>[22x]MAALIAENFRFLSLFFKSKDVMIFNGLVALGTVGSQELFSVVAFHCPCSPARNYLYGLAAIGVPALVLFIIGIILNNHTWNLVAECQHRRTKNCSAAPTFLLLSSILGRAAVAPVTWSVISLLRGEAYVCALSEFVDPSSLTAREEHFPSAHATEILARFPCKENPDNLSDFREEVSRRLRYESQLFGWLLIGVVAILVFLTKCLKHYCSPLSYRQEAYWAQYRANEDQLFQRTAEVHSRVLAANNV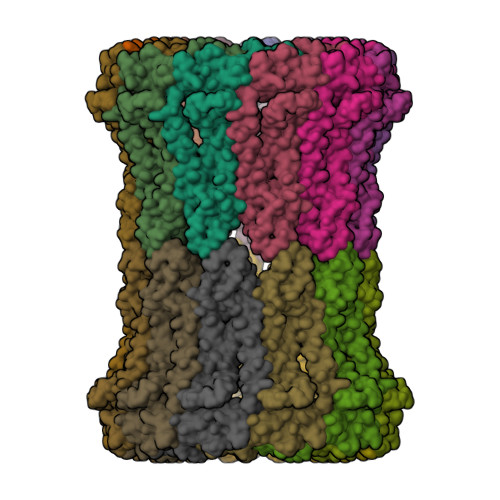RRFFGFVALNKDDEELIANFPVEGTQPRPQWNAITGVYLYRENQGLPLYSRLHKWAQGLAGNGAAPDNVEMALLPSFESRLVPR>MTTNYIFVTGGVVSSLGKGIAAASLAAILEARGLNVTIMKLDPYINVDPGTMSPIQHGEVFVTEDGAETDLDLGHYERFIRTKMSRRNNFTTGRIYSDVLRKERRGDYLGATVQVIPHITNAIKERVLEGGEGHDVVLVEIGGTVGDIESLPFLEAIRQMAVEIGREHTLFMHLTLVPYMAASGEVKTKPTQHSVKELLSIGIQPDILICRSDRAVPANERAKIALFCNVPEKAVISLKDVDSIYKIPGLLKSQGLDDYICKRFSLNCPEANLSEWEQVIFEEANPVSEVTIGMVGKYIELPDAYKSVIEALKHGGLKNRVSVNIKLIDSQDVETRGVEILKGLDAILVPGGFGYRGVEGMITTARFARENNIPYLGICLGMQVALIDYARHVANMENANSTEFVPDCKYPVVALITEWRDENGNVEVRSEKSDLGGTMRLGAQQCQLVDDSLVRQLYNAPTIVERHRHRYEVNNMLLKQIEDAGLRVAGRSGDDQLVEIIEVPNHPWFVACQFHPEFTSTPRDGHPLFAGFVKAASEFQKRQA[4x]

Cytidine triphosphate synthase (CTPS) plays a critical role in catalyzing the final and rate‐limiting step of de novo cytidine triphosphate (CTP) synthesis. CTPS is composed of a glutamine amidotransferase (GAT) domain and a kinase‐like ammonia ligase (AL) domain 1 , 2 . It utilizes ammonia generated from glutamine and adenine triphosphate (ATP) as an energy source to convert the substrate uridine triphosphate (UTP) into CTP 3 . Filaments of CTPS have been confirmed and characterized in multiple species and conditions, where ecCTPS has been shown to form large‐scale inhibitory filaments in the presence of product CTP 20 .

Utilizing cryo‐EM and single particle analysis, we resolved the structure of purified ecCTPS bounded with CTP, NADH, and DON, achieving a resolution of 2.9 Å. The results of the two‐dimensional (2D) classification provided a clear visualization of the ecCTPS filament, wherein it assembles into filaments with CTPS tetramers as the helical unit. In our obtained structure, DON forms a covalent bond with C379, a residue that is critical for the catalytic function of ecCTPS. Upon the conjunction of DON, the GAT domain adopts a closed conformation, preventing external NH4 + from accessing the ammonia tunnel through the catalytic pocket of GAT for further utilization by the AL domain. Through computational analysis, we observed the presence of a solvent‐accessible channel on the side of F353 close to the AL domain, connecting an internal cavity within the GAT domain. The existence of this entrance to the ammonia tunnel explains the feasibility of ecCTPS utilizing NH4 + as a substrate when DON is bound to the GAT pocket. In our structure of ecCTPS, CTP binding was observed in the UTP binding pocket, consistent with previously resolved ecCTPS–CTP complexes 18 , 21. Aligning the structure with those of dmCTPS and hCTPS containing nonclassical CTP binding, we identified a clash between the CTP portion of the eukaryotic CTPS model and the solvent‐accessible surface of the ecCTPS model due to hindrance by amino acids H75 and I20. We observed NADH binding in the ATP binding pocket in our model. At the 1σ counter level, the adenine portion of NADH displayed clear and distinct density, while the remaining portion lacked stable density.> AERPTLPIPDLLTTDARNRIQLTIGAGQSTFGGKTATTWGYNGNLLGPAVKLQRGKAVTVDIYNQLTEETTLHWHGLEVPGEVDGGPQGIIPPGGKRSVTLNVDQPAATCWFHPHQHGKTGRQVAMGLAGLVVIEDDEILKLMLPKQWGIDDVPVIVQDKKFSADGQIDYQLDVMTAAVGWFGDTLLTNGAIYPQHAAPRGWLRLRLLNGCNARSLNFATSDNRPLYVIASDGGLLPEPVKVSELPVLMGERFEVLVEVNDNKPFDLVTLPVSQMGMAIAPFDKPHPVMRIQPIAISASGALPDTLSSLPALPSLEGLTVRKLQLSMDPILDMMGMQMLMEKYGDQAMAGMDHSQMTSFAEYWALLSMNHGGKFDFHHANKINGQAFDMNKPMFAAAKGQYERWVISGVGDMMLHPFHIHGTQFRILSENGKPPAAHRAGWKDTVKVEGNVSEVLVKFNHDAPKEHAYMAHCHLLEHEDTGMMLGFTVKDPNSSSVDKLAAALEHHHHH

CueO plays an important role in copper homeostasis by oxidation of toxic cuprous ions to cupric ions. As with all multi-copper oxidases, it contains four copper atoms distributed within one type 1 (T1)2 copper site and a trinuclear cluster comprising the T2 and T3 copper sites. A distinguishing feature of CueO is a partially structured 45-amino acid segment (residues 356–404) capping the entrance to the T1/sCu copper-binding sites. The goal of the current study was to engineer the highly compliant MRS such that CueO activity would be modulated by engagement of a partner protein with a scaffolded peptide.

Having delineated the MRS subregion suitable for introduction of peptide sequences, we produced two additional constructs (CueO-PMI and CueO-PM2) using previously identified higher-affinity MDM2 binding peptides. The affinity of these variants for recombinant MDM2 (residues 6–125 comprising the p53 binding domain) was first measured by fluorescence polarization. Both variants showed high affinity to MDM2 (apparent Kd 28 ± 1 and 25 ± 1.5 nm, respectively), comparable with affinities of their unmodified linear and stapled versions. Whereas the activities of CueO and CueO-HA were similar, CueO-PM2 showed ∼2-fold reduced activity, indicating auto-inhibition by the PM2 peptide that is relieved upon MDM2 interaction. The reduced activity of CueO-PM2 compared with CueO and CueO-HA along with its impaired Cu binding suggests that in the absence of MDM2, the PM2 helix reorients itself to block access to the sCu and T1 binding sites, most likely by packing adjacent to the CueO α5 helix. However, in the highly similar structures of CueO-PM2 and CueO-12.1 (Cα RMSD = 0.22 Å), the MRS-PM2/12.1 regions were not resolved. The rest of the CueO-PM2 structure showed high similarity to both the MDM2-bound form (Cα RMSD = 0.3 Å) and native CueO (Cα RMSD = 0.37 Å). As the PM2-containing MRS retains some intrinsic disorder, a transient conformation likely inhibits CueO function, with all or a subset of the Phe, Trp, and Leu residues in PM2 contributing significantly. The reduced T1 copper occupancy observed in CueO-PM2 likely accounts for its reduced kcat, with this phenotype contingent on either all or a subset of the Phe/Trp/Leu residues in the PM2 insert. In agreement, CueO-PM2 meets this criterion (kcat CueO-PM2/kcat CueO = 0.32), and MDM2 binding results in increased activity.The TWIK-related Halothane Inhibited K+ channel (THIK1), named for the early observation that halothane and other volatile anesthetic (VA) agents inhibit THIK1 currents (1), is a K2P channel expressed in microglia (2), primary immune cells of the central nervous system (CNS). pmcTandem pore domain (K2P) potassium channels play vital roles across human physiology, conducting noninactivating potassium currents that set cellular resting membrane potentials. In response to inflammatory or infectious neuronal cues, THIK1 mediated efflux of potassium ions from the microglial cytoplasm modulates activation of the NLRP3 inflammasome and pharmacologic or genetic disruption of THIK1 activity decreases inflammasome-mediated production of the proinflammatory cytokine IL-1β. The overall structure of the THIK1 channel follows the canonical K2P architecture, featuring a dimeric channel assembly with a domain-swapped cap domain at the extracellular face of the channel, positioned above a central pore formed by the TM2 and TM4 helices.

To facilitate cryo-EM structure determination and anesthetic photolabeling studies, we purified a C-terminally truncated version of THIK1 (KCNK13), bearing residues 1 to 309 of the THIK1 protein sequence. Using cryo-EM, we solved a 3.2 Å structure of this THIK1EM channel construct. Our 3.2 Å THIK1 structure is in a putative closed conformation, due to the presence of an occlusive pore gate constituted by a pair of inward-facing TM4 tyrosine residues positioned directly below the potassium selectivity filter. Inwardly opposed Tyr273 sidechains arise from the pore-lining TM4 helixes and meet within the pore to form a central occlusive constriction ~6 Å below the THIK1 selectivity filter. In the presumed closed conformation we observe in the THIK1 structure, the Y-gate tyrosine residues limit the size of the ion conduction pathway to a diameter of less than 2 Å, precluding passage of potassium ions to the selectivity filter and dividing the inner pore into a large lower vestibule and a much smaller hydrophilic chamber directly below the selectivity filter. The cap domain of THIK1 contains two predicted N-glycosylation sites at Asp59 and Asp65 and in our THIK1 cryo-EM map we observe density consistent with glycosylation of both sites. Consistent with this notion, we observe EM density between the S4 selectivity filter Thr110 and Thr237 residues and the Y-gate in our cryo-EM map of THIK1. This “S5” site density is equivalently spaced and linearly aligned with the S1 to S4 potassium ion binding sites, and we therefore modeled this density as a potassium ion. A five-residue sequence, from Gly189 to Ser193, crosses the distal TM2 helix and adopts an inward-facing orientation previously unobserved in other K2P structures. In the THIK1 cryo-EM density map, we find a curved lipid-like density buried within the core of the THIK1 protein, directly behind the selectivity filter.

>[2x]MAGRGFSWGPGHLNEDNARFLLLAALIVLYLLGGAAVFSALELAHERQAKQRWEERLANFSRGHNLSRDELRGFLRHYEEATRAGIRVDNVRPRWDFTGAFYFVGTVVSTIGFGMTTPATVGGKIFLIFYGLVGCSSTILFFNLFLERLITIIAYIMKSCHQRQLRRRGALPQESLKDAGQCEVDSLAGWKPSVYYVMLILCTASILISCCASAMYTPIEGWSYFDSLYFCFVAFSTIGFGDLVSSQNAHYESQGLYRFANFVFILMGVCCIYSLFNVISILIKQSLNWILRKMDSGCCPQCQRGLLRS> MAEDKSKRDS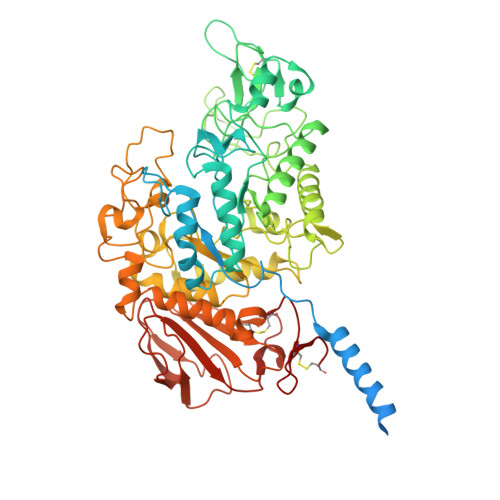IEMSMKGCQTNNGFVHNEDILEQTPDPGSSTDNLKHSTRGILGSQEPDFKGVQPYAGMPKEVLFQFSGQARYRIPREILFWLTVASVLVLIAATIAIIALSPKCLDWWQEGPMYQIYPRSFKDSNKDGNGDLKGIQDKLDYITALNIKTVWITSFYKSSLKDFRYGVEDFREVDPIFGTMEDFENLVAAIHDKGLKLIIDFIPNHTSDKHIWFQLSRTRTGKYTDYYIWHDCTHENGKTIPPNNWLSVYGNSSWHFDEVRNQCYFHQFMKEQPDLNFRNPDVQEEIKEILRFWLTKGVDGFSLDAVKFLLEAKHLRDEIQVNKTQIPDTVTQYSELYHDFTTTQVGMHDIVRSFRQTMDQYSTEPGRYRFMGTEAYAESIDRTVMYYGLPFIQEADFPFNNYLSMLDTVSGNSVYEVITSWMENMPEGKWPNWMIGGPDSSRLTSRLGNQYVNVMNMLLFTLPGTPITYYGEEIGMGNIVAANLNESYDINTLRSKSPMQWDNSSNAGFSEASNTWLPTNSDYHTVNVDVQKTQPRSALKLYQDLSLLHANELLLNRGWFCHLRNDSHYVVYTRELDGIDRIFIVVLNFGESTLLNLHNMISGLPAKMRIRLSTNSADKGSKVDTSGIFLDKGEGLIFEHNTKNLLHRQTAFRDRCFVSNRACYSSVLNILYTSC>[2x]MTRRIRIGGAQMGAISRSDSKKEIVDRLI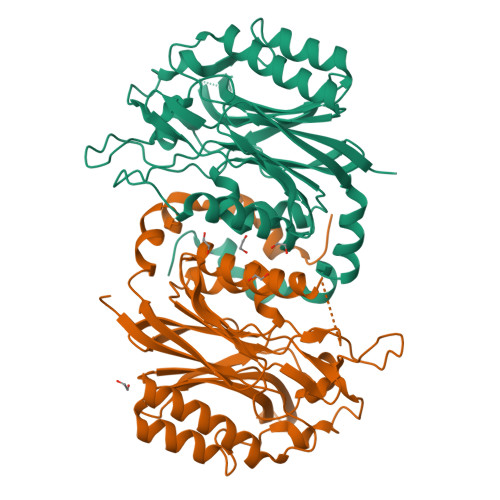ALLRQASEKGCELVVFPELALSTFFPRWYAERDGMDGYFEDGMPNAATLPLFEEARRLGIGFSLGYAELVQEDGRVRRFNTTVLVERNGEIVGKYRKIHLPGHAEYEPERSHQHLEKRYFEVGNTGFQVWDAFGGRVGMAICNDRRWVETYRVMGLQDVELILIGYNTPVADSLSGESETLGMFHNHLTMQAGAYQNSTWVVGVAKAGVEDGHRLMGGSVIVAPTGEIVAQAMTEGDELIVADCDLDRCRYYKSHIFNFAAHRRPEFYQRITSQTGVE> MAPSRANTKVIVVGGGGTIGSSTALHLVRSGYTPSNVTVLDAYPIPSSQSAGNDLNKIMDADADPAADAARQMWNEDELFKKFFHNTGRLDCAHGEKDIADLKKRYQNLVDWGLDATVEWLDSEDEILKRMPQLTRDQIKGWKAIFSKDGGWLAAAKAIKAIGEYLRDQGVRFGFYGAGSFKQPLLAEGVCIGVETVDGTRYYADKVVLAAGAWSPTLVELQEQCVSKAWVYGHIQLTPEEAARYKNSPVVYNGDVGFFFEPNEHGIIKVCDEFPGFTRFKMHQPFGAKAPKRISVPRSHAKHPTDTIPDASIVRIRRAIATFMPQFKNKPLFNQAMCWCTDTADGHLLICEHPEWKNFYLATGDSGDSFKLLPIIGKYVVELLEGTLADELAHKWRWRPGSGDALKSRR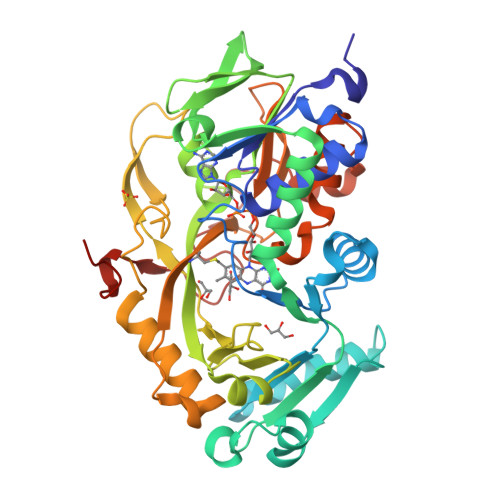EAPAKDLADMPGWNHDHHHHHH>[2x]QSNAIWGLDRIDQRNLPLDRNYNANFDGFGVTAYVIDTGVNNNHEEFGGRSVSGYDFVDNDADSSDCNGHGTHVAGTIGGSQYGVAKNVNIVGVRVLSCSGSGTTSGVISGVDWVAQNASGPSVANMSLGGGQSTALDSAVQGAIQSGVSFMLAAGNSNADACNTSPARVPSGVTVGSTTSSDSRSSFSNWGSCVDLFAPGSQIKSA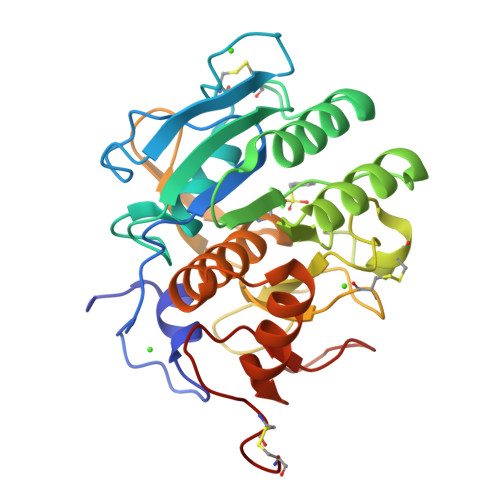WYDGGYKTISGTSMATPHVAGVAALYLQENNGLTPLQLTGLLNSRASENKVSDTRGTTNKLLYSLADSGCEPDCGGP>CGGGCG[2x];>CGCCCG[2x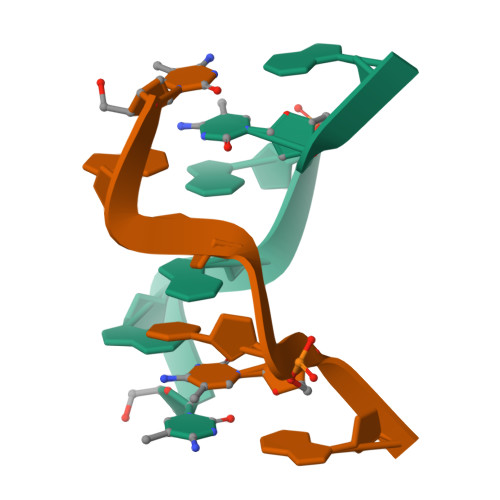]> MTGGLVLNAISRAGGAMGGLGLIKSLAEKEKQLLERLEAAKKEAEERVKRA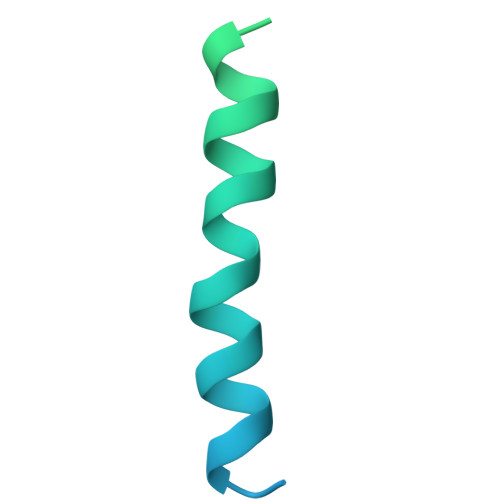EAEAKALLEEAEAKAKALEAQYRERERAETEALLARYRERAEAEAKAVREKAMARLDEAVALVLKEVLP> GSMDPTAGSKKEPGGGAATEEGVNRIAVPKPPSIEEFSIVKPISRGAFGKVYLGQKGGKLYAVKVVKKADMINKNMTHQVQAERDALALSKSPFIVHL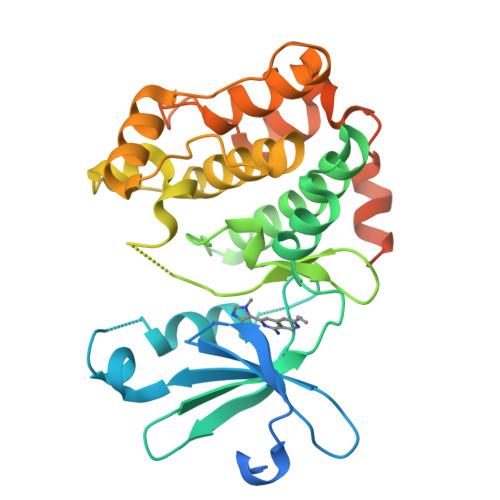YYSLQSANNVYLVMEYLIGGDVKSLLHIYGYFDEEMAVKYISEVALALDYLHRHGIIHRDLKPDNMLISNEGHIKLTDFGLSKVTLNRDINMMDILTTPRTFCILGTPDYLAPELLLGRAHGPAVDWWALGVCLFEFLTGIPPFNDETPQQVFQNILKRDIPWPEGEEKLSDNAQSAVEILLTIDDTKRAGMKELKRHPLFSDVDWENLQHQTMPFIPQPDDETDTSYFEARNTAQHLTVSGFSL> PVSEKQLAEVVANTITPLMKAQSVPGMAVAVIYQGKPHYYTFGKADIAANKPVTPQTLFELGSISKTFT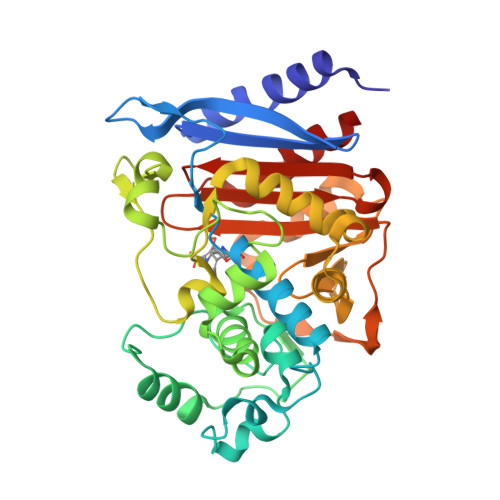GVLGGDAIARGEISLDDAVTRYWPQLTGKQWQGIRMLDLATYTAGGLPLQVPDEVTDNASLLRFYQNWQPQWKPGTTRLYANASIGLFGALAVKPSGMPYEQAMTTRVLKPLKLDHTWINVPKAEEAHYAWGYRDGKAVRVSPGMLDAQAYGVKTNVQDMANWVMANMAPENVADASLKQGIALAQSRYWRIGSMYQGLGWEMLNWPVEANTVVEGSDSKVALAPLPVAEVNPPAPPVKASWVHKTGSTGGFGSYVAFIPEKQIGIVMLANTSYPNPARVEAAYHILEAL> MGSDKIHHHHHHENLYFQGQRFEIQQH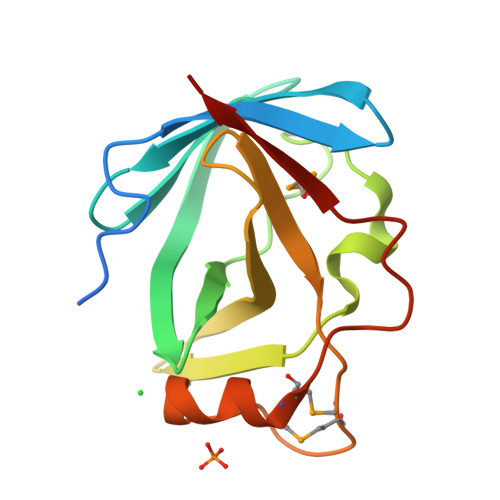NETIGSIYFSADYAHIRGIEKGTAKYFIDKVGSKRYLFIEYIPDNVLNCKPDFWKTLKYKKDKVTYYVYLIENLDDEVFHLSALQDMNRIPIDIADDVATMGKSPHQNDRMTLKLNKNN> MDKGKSVKSTEKSVGMPPKTPKTDNNAHVDNEFLILQVNDAVFPIGSYTHSFGLETYIQQKKVTNKESALEYLKANLSSQFLYTEMLSLKLTYESALQQDLKKILGVEEVIMLSTSPMELRLANQKLGNRFIKTLQAMNELDMGEFFNAYAQKTKDPTHATSYGVFAASLGIE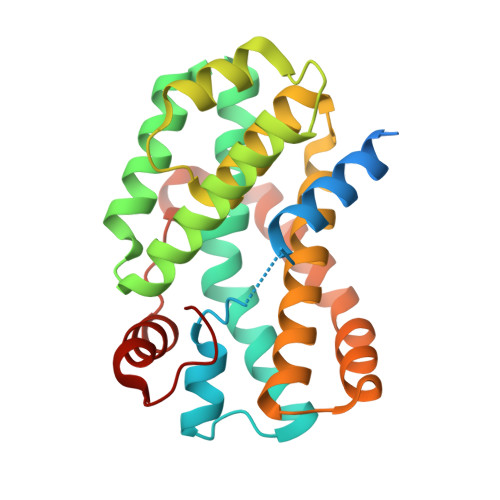LKKALAHYLDAQTSNMVINCVKSVPLSQNDGQKILLSLQSPFNQLIEKTLELDESHLCTASVQNDIKAMQHESLYSRLYMS> MDFLSNFL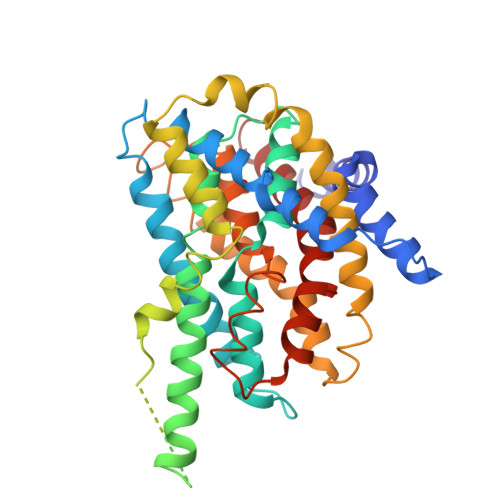TDFVGQLQSPTLAFLIGGMVIAALGTQLVIPEAISTIIVFMLLTKIGLTGGMAIRNSNLTEMLLPVAFSVILGILIVFIARFTLAKLPNVRTVDALATGGLFGAVSGSTMAAALTTLEESKISYEAWAGALYPFMDIPALVTAIVVANIYLNKRKRKSAAASIEESFSKQPVAAGDYGDQTDYPRTRQEYLSQQEPEDNRVKIWPIIEESLQGPALSAMLLGLALGIFTKPESVYEGFYDPLFRGLLSILMLIMGMEAWSRIGELRKVAQWYVVYSLIAPIVHGFIAFGLGMIAHYATGFSLGGVVVLAVIAASSSDISGPPTLRAGIPSANPSAYIGSSTAIGTPIAIGVCIPLFIGLAQTLGAG>MTESQSYETRQARPAGQSLAERVARLVAIDPQAAAAVPDKAVAERATQQGLRLAQRIEAFLSGYGDRPALAQRAFEITKDPITGRAVATLLPKFETVSYRELLERSHAIASELANHAEAPVKAGEFIATIGFTSTDYTSLDIAGVLLGLTSVPLQTGATTDTLKAIAEETAPAVFGASVEHLDNAVTTALATPSVRRLLVFDYRQGVDEDREAVEAARSRLAEAGSAVLVDTLDEVIARGRALPRVALPPATDAGDDSLSLLIYTSGSTGTPKGAMYPERNVAQFWGGIWHNAFDDGDSAPDVPDIMVNFMPLSHVAGRIGLMGTLSSGGTTYFIAKSDLSTFFEDYSLARPTKLFFVPRICEMIYQHYQSELDRIGAADGSPQAEAIKTELREKLLGGRVLTAGSGSAPMSPELTAFIESVLQVHLVDGYGSTEAGPVWRDRKLVKPPVTEHKLIDVPELGYFSTDSPYPRGELAIKTQTILPGYYKRPETTAEVFDEDGFYLTGDVVAEVAPEEFVYVDRRKNVLKLSQGEFVALSKLEAAYGTSPLVRQISVYGSSQRSYLLAVVVPTPEALAKYGDGEAVKSALGDSLQKIAREEGLQSYEVPRDFIIETDPFTIENGILSDAGKTLRPKVKARYGERLEALYAQLAETQAGELRSIRVGAGERPVIETVQRAAAALLGASAAEVDPEAHFSDLGGDSLSALTYSNFLHEIFQVEVPVSVIVSAANNLRSVAAHIEKERSSGSDRPTFASVHGAGATTIRASDLKLEKFLDAQTLAAAPSLPRPASEVRTVLLTGSNGWLGRFLALAWLERLVPQGGKVVVIVRGKDDKAAKARLDSVFESGDPALLAHYEDLADKGLEVLAGDFSDADLGLRKADWDRLADEVDLIVHSGALVNHVLPYSQLFGPNVVGTAEVAKLALTKRLKPVTYLSTVAVAVGVEPSAFEEDGDIRDVSAVRSIDEGYANGYGNSKWAGEVLLREAYEHAGLPVRVFRSDMILAHRKYTGQLNVPDQFTRLILSLLATGIAPKSFYQLDATGGRQRAHYDGIPVDFTAEAITTLGLAGSDGYHSFDVFNPHHDGVGLDEFVDWLVEAGHPISRVDDYAEWLSRFETSLRGLPEAQRQHSVLPLLHAFAQPAPAIDGSPFQTKNFQSSVQEAKVGAEHDIPHLDKALIVKYA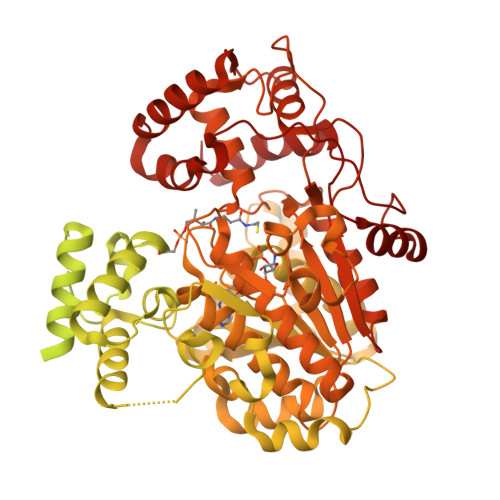EDIKQLGLL[4x]>[2x]MIQGVIQKIAGPAVIAKGMLGARMYDISKVGEEGLVGEIIRLDGDTAFVQVYEDTSGLKVGEPVVSTGLPLAVELGPGMLNGIYDGIQRPLERIREKTGIYITRGVVVHALDREKKWAWTPMVKPGDEVRGGMVLGTVPEFGFTHKILVPPDVRGRVKEVKPAGEYTVEEPVVVLEDGTELKMYHTWPVRRARPVQRKLDPNTPFLTGMRILDVLFPVAMGGTAAIPGPFGSGKSVTQQSLAKWSNADVVVYVGSGERGNEMTDVLVEFPELTDPKTGGPLMHRTVLIANTSNMPVAAREASIYVGVTIAEYFRDQGFSVALMADSTSRWAEALREISSRLEEMPAEEGYPPYLAARLAAFYERAGKVITLGGEEGAVTIVGAVSPPGGDMSEPVTQSTLRIVGAFWRLDASLAFRRHFPAINWNGSYSLFTSALDPWYRENVAEDYPELRDAISELLQREAGLQEIVQLVGPDALQDAERLVIEVGRIIREDFLQQNAYHEVDAYSSMKKAYGIMKMILAFYKEAEAAIKRGVSIDEILQLPVLERIGRARYVSEEEFPAYFEEAMKEIQGAFKALA;>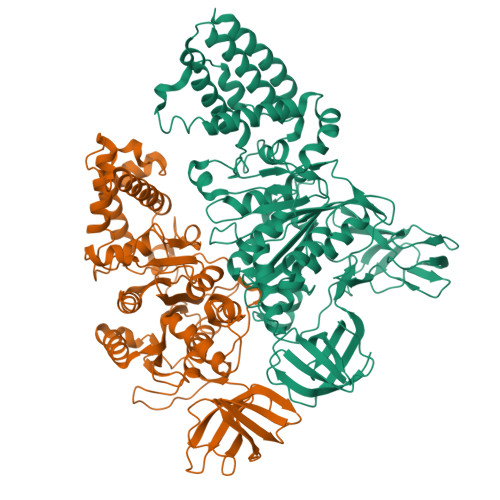[2x]MDLLKKEYTGITYISGPLLFVENAKDLAYGAIVDIKDGTGRVRGGQVIEVSEEYAVIQVFEETTGLDLATTSVSLVEDVARLGVSKEMLGRRFNGIGKPIDGLPPITPEKRLPITGLPLNPVARRKPEQFIQTGISTIDVMNTLVRGQKLPIFSGSGLPANEIAAQIARQATVRPDLSGEGEKEEPFAVVFAAMGITQRELSYFIQEFERTGALSRSVLFLNKADDPTIERILTPRMALTVAEYLAFEHDYHVLVILTDMTNYSEALREIGAAREEIPGRRGYPGYMYTDLATIYERAGVVEGKKGSVTQIPILSMPDDDRTHPIPDLTGYITEGQIQLSRELHRKGIYPPIDPLPSLSRLMNNGVGKGKTREDHKQVSDQLYSAYANGVDIRKLVAIIGEDALTENDRRYLQFADAFERFFINQGQQNRSIEESLQIAWALLSMLPQGELKRISKDHIGKYYG> GPLGSSSENKID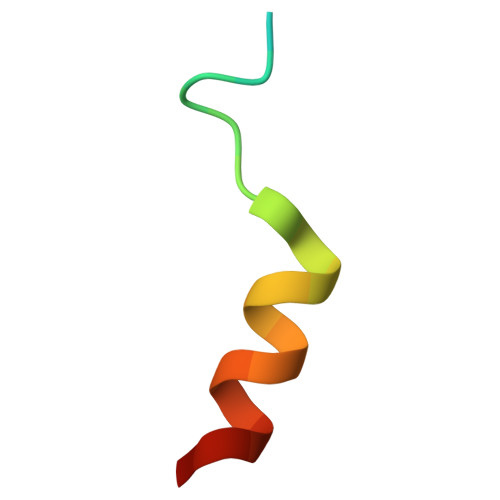FNDFIKRLKTGK>MAECSVDIQGNDQMQFNTNAITVDKSCKQFTVNLSHPGNLPKNVMGHNWVLSTAADMQGVVTDGMASGLDKDYLKPDDSRVIAHTKLIGS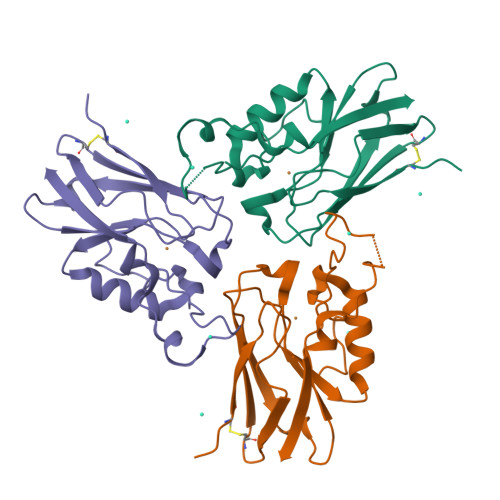GEKDSVTFDVSKLKEGEQYMFFCTFSGYIDTNNDGWIEGDELYSPGHSALMKGTLTLK[3x]> STGSKQRSQNRSKTPKNQEALRMANVAENSSSDQRQACKKHELYVSFRDLGWQDWIIAPEGYAAY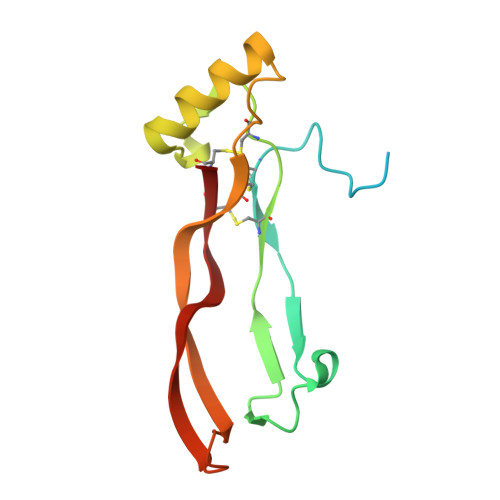YCEGECAFPLNSYMNATNHAIVQTLVHFINPETVPKPCCAPTQLNAISVLYFDDSSNVILKKYRNMVVRACGCH>MGKITLYEDRGFQGRHYECSSDHTNLQPYLSRCNSASVDSGCWMLYEQPNYSGLQYFLRRGDYADHQQWMGLSDSVRSCRLIPHSGSHRIRLYEREDYRGQMIEFTEDCSCLQDRFRFNEIHSLNVLEGSWVLYELSNYRGRQYLLMPGDYRRYQDWGATNARVGSL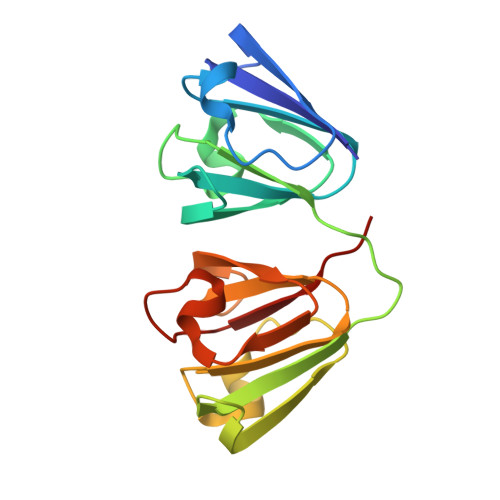RRVIDFS[2x]> SMLDDAKARLRKYDIGGKYSHLPYNKYSVLLPLVAKEGKLHLLFTVRSEKLRRAPGEVCFPGGKRDPTDMDDAATALREAQEEVGLRPHQVEVVCCLVPCLIDTDTLITPFVGLIDHNFQAQPNPAEVKDVFLVPLAYFLHPQVHDQHYVTR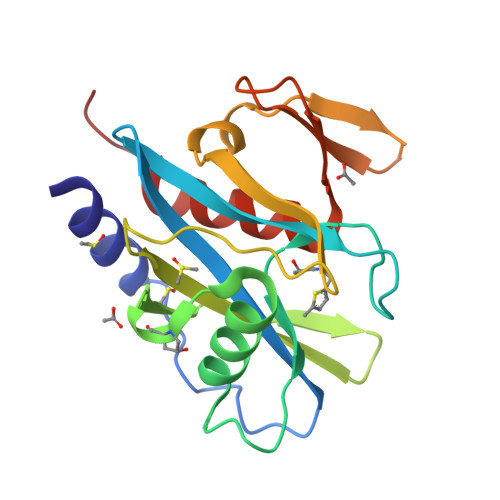LGHRFINHIFEYTNPEDGVTYQIKGMTANLAVLVAFIILEKKPT>[2x]GGDPHMMFGKKKNNGGSSTARYSAGNKYNTLSNNYALSAQQLLNASKIDDIDSMMGFERYVPPQYNGRFDAKDIDQIPGRVGWLTNMHATLVSQETLSSGSNGGGNSNDGERVTTNQGISGVDFYFLDEEGGSFKSTVVYDPYFFIACNDESRVNDVEELVKKYLESCLKSLQIIRKEDLTMDNHLLGLQKTLIKLSFVNSNQLFEARKLLRPILQDNANNNVQRNIYNVAANGSEKVDAKHLIEDIREYDVPYHVRVSIDKDIRVGKWYKVTQQGFIEDTRKIAFADPVVMAFDIETTKPPLKF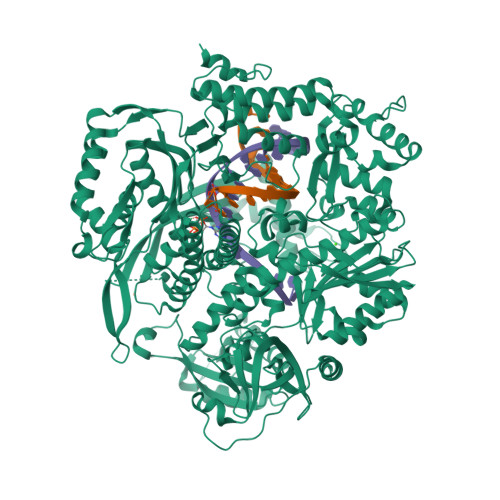PDSAVDQIMMISYMIDGEGFLITNREIISEDIEDFEYTPKPEYPGFFTIFNENDEVALLQRFFEHIRDVRPTVISTFNGDFFDWPFIHNRSKIHGLDMFDEIGFAPDAEGEYKSSYCSHMDCFRWVKRDSYLPQGSQGLKAVTQSKLGYNPIELDPELMTPYAFEKPQHLSEYSVSDAVATYYLYMKYVHPFIFSLCTIIPLNPDETLRKGTGTLCEMLLMVQAYQHNILLPNKHTDPIERFYDGHLLESETYVGGHVESLEAGVFRSDLKNEFKIDPSAIDELLQELPEALKFSVEVENKSSVDKVTNFEEIKNQITQKLLELKENNIRNELPLIYHVDVASGYPNIMTTNRLQPDSIKAERDCASCDFNRPGKTCARKLKWAWRGEFFPSKMDEYNMIKRALQNETFPNKNKFSKKKVLTFDELSYADQVIHIKKRLTEYSRKVYHRVKVSEIVEREAIVCQRENPFYVDTVKSFRDRRYEFKGLAKTWKGNLSKIDPSDKHARDEAKKMIVLYDSLQLAHKVILNSFYGYVMRKGSRWYSMEMAGITCLTGATIIQMARALVERVGRPLELDTDGIWCILPKSFPETYFFTLENGKKLYLSYPCSMLNYRVHQKFTNHQYQELKDPLNYIYETHSENTIFFEVDGPYKAMILPSSKEEGKGIKKRYAVFNEDGSLAELKGFELKRRGELQLIKNFQSDIFKVFLEGDTLEGCYSAVASVCNRWLDVLDSHGLMLEDEDLVSLICENRSMSKTLKEYEGQKSTSITTARRLGDFLGEDMVKDKGLQCKYIISSKPFNAPVTERAIPVAIFSADIPIKRSFLRRWTLDPSLEDLDIRTIIDWGYYRERLGSAIQKIITIPAALQGVSNPVPRVEHPDWLKRKIAT> MGSSHHHHHHSSGLVPRGSHSEQKLISEEDLSMASISKDFTNLLNTLIDGQIGAASRQTEWFNMSPDERTDYIKQVDERLQEMQQSTLSVLAAQHFQMQDNPVSVGDQLQTLQKRRQQMTDVPGTPAINAYKQQLDRDILLYRRQQTAMTHFDSTWRKVLVMLGPDDSKPLNATTLRENAVDKQAKLDTEIKRLEQQLTIQVADSTFSQKYVTLFSELQAYKDVNARYNALLKASATEEAAALGALTKVPQASDDLPVNISLLMMEERPGYIRMNVALVNASTDGRFKDFFLENGRLVVLTDGVLNFSFGTAARSLAWQQQYRLKSEPPSFRSPTYTPIRSVLVKTEFVEKYFANYLVSESTLRGGFKAQLLGNGRKMLLTSVDRKVPNQIGIQVSGQAPNTTITREVPLASALSDLINQNADIASFRTIGLEGFRQSSYHPDRDGLFVNIHELERSVGFAGRQYLLEMPQDNDYLSATPFGVMSVDGDKVSSSHLSKAQTDTLYQYNAAFFEKLEQLRSGGMKASRLFEGSIERTAFVQQLVRLLERNHITPAGVLAPEYPRDNMRDIKGNNLNKVLWEQAFAASVWRSRDNDPLLFRLATRLVKNPAVVKVLQNGYVQSDIAQARELLAPLYEQWRTRAVEAETQRVASANAAQHPSNPKVHVFDQAEVERSLDDKLLILLLTGPQSLEGTDVQLRPMVEAALLSNEGRSLRKQILFHALRPVADSFSKAAAPVNPHAELGVGKIMINNRLNQPDPYLILNTSSEEQAYRDGSYLIKDDKYRSYNQFRPDFKNDATRYMNDLDTPFVGGISGTTQTVSNVLTELFGGALSVKQYWQFQMANAAFMIRNGYHSFFETFYVAARYEPEGADSIGKEMLQMFDKYRVEGSKKALQGKLYDGVMARVLPIINQGLSAADEFHPPRFTRIGPRPALLGQAVKDLELKAGLTSVGDGFEPRQGSADIHQFVTDPVLFAKTHTVSAEALVRSGRLPAEGSAQLVKVGSGLYELEYTEQSANDISSSSIPAYFLGYNGPNQANAVPAYVDIPKRTIAGNFLFTGTLSGGSLVVTSLDANTFRVYHDGRVNSSLLYDNVVMAVDYKDYQIAGTAEGLAAAYMQYVNHEWQLVLQRQEYQRDGQMLRLRLRDDEEPLSIQVADSQVVERNQAQFVAYREQIHQQLKKVATQFEVSISGVSDGVYTEGEFSPDHPAIAAWAKLCAEVYDRINADTKQLVDKRNKLYENRRNTIRRDLINQQIKQLNITLEYYKAQYDTVLREAGFVEQSWLWQQIKAKNGSAAVVRIDDTAIQGGGKQRTDSVGERYAISEAYQRGARGTGFSDGLRNFREIEIPGVDDKMSALEMKRLFLEGKLTSEQQGALSGRITETSRAEYIDKVLRQTAVFSEDFHDAGSVFDRLVPQDFYLSLVGDRSGGRCYPLVRAMTVALASGGEAGINSLVQKLFFASADPQAGSSTLLRNSLIKLHSNVEAVQASTELGQFGLSEVVSRLAATTGTSMFALNTQNHSMMVGSTVTTEGRRYYFYDPNVGIFAFDNTKSLSRAMEQHLVGRRLAVHYGSFGSKSAPAFNLIEIDTGKMAEVPVGNGLNVADLTRFEELSSVIGQRRQVEQVMSAQERITEDLQLSTALQAFDAEQWGARFEAASTRLAQEHQLDSRWLPIIATTEEQGEGRYRVQFINRDQPEQTRWLDTDDSTFVEFRRFVDEHMSVLNEHFTLESGRMRPRGGVGEAAPVDGLNAGFAVQALIQWFSDKNRHDAANGMASPDLATALKVHSYLNFVQMVHGGVQDVIKVTALVRTALRGEVVAAQTSFKEFALSLGHTVNEGVGVLFGGAMIGLDAYELAHAENDVQKAVFGTQLAFDSASFVTGAAGIGAGLVGASTAGAVLGGAGVILGGLAVGFTALAQAFGAVAEDAKAVGRYFDTVDKAYKGNGYRYDNEKQVLVPLAGAVIKTLDLSKNQIDFDSQYIYRTHSGSTGSGKINYFFWVGDFPRMVHDRGQAIEVRSGIGYKDVSRPLEHGDSNVVILPGTPKSYISYEYMLLPGATTRHDAGFDVIRRLEEDKRFDYDFYIFPGEETIRRIHHEYVDTPIEVVLDQRNRQLVAPELPKELHGFLCYEIKGAGGEYLIGLNEGAKVNLTSDVASTWIIDSSQLASDSISVSKDQLLVGEKGKEVVVKLYLAQNSQVLVVNGKGEVRKVDFTSLTAQVISEDASKWQVPGQQIEQHLSDLAKAHQLHGQYVVVENYRHQGRDVGRAFYDVTKDRMLFTDTTNEQAKRAQLGAVMGDYAYFYDADNAVAWRVDIATGQVDAQFEPWFNQNAGHISRFWQEGDVVYLARRYRLKEREAELGYRIIGDRMELVSAVGDDALLQLSARIGRHGDELEAILQGYRSNSTQRGTLMYTLGARLIQPTSAALVTVFGVDAAGVPHRYWIRTSDGTLIKPNLAPPADQTLHFEAHEQTRSAWQIPADLVLAGSMPLLGGKEVFFFYSKEQKTLFRQEGPGQEVLDANQPSALRVTTPALTNVINLNGHLVVVTEDGRVARLDALGQLSYAAVNEHWLKGRIHWWQDLTSVTDGRATLAVFGVKDTDGKSLLPVWYHNGQVVVASAALQDKHPQFLGFEVDGSSARLFEPASGKLYRQPAMTADALAAAFGTDEVLEASAQLPAANELEPELHLKAAEQVDAGLRLTTVKGEILLRTHDGKLQLVAVDKDWQQDNLVRLSQALAEVAGQWRVKGVLTLQGDDTQGWFDVGSGQVFSIGGIPATDNLRFIGIAVGKKGAYVYNPTDQMLYQVKESGAQKLNHYADVERIGSSLLLQDGGKGDLSPMLIAGVDSVVLHGGAGSDTYRLSQTMWSYYRTVVIDNDDPNQVLDRLIILAVDAEKIFVSRHEDDLMLTDSVNGTVLVIRKVFGSQAVTHRHLQIDLEGSSSVISVDHLVKGFTRLGTANIGLFELPWAIELDYKDDDDK

The bacterial Makes caterpillars floppy 1 (Mcf1) toxin promotes apoptosis in insects, leading to loss of body turgor and death. The structure reveals that Mcf1 is divided into an N-terminal head region and a C-terminal tail region. The head contains an N-terminal effector domain (NED), an activator-binding domain (ABD), and a protease effector domain (PED). The tail consists of two putative translocation and three putative receptor-binding domains.

To understand how Mcf1 is built in molecular detail, we heterologously expressed and purified the full-length Mcf1 complex from Photorhabdus luminescens and determined its structure using single particle cryo-EM to 3.6 Å resolution. Since the toxin proved to be inherently flexible, we performed a series of signal subtraction and local refinements of subregions of the complex. The resulting composite reconstruction allowed us to build 92% of the Mcf1 atomic model de novo. The structure reveals that Mcf1 is a monomeric, asymmetric protein. Based on its overall shape, reminiscent of a seahorse, it can be divided into two parts - an N-terminal head and a C-terminal tail region. In addition, we noticed a large spherical density of 10 Å diameter in the middle of the head that is coordinated by five arginines from all three head domains. Its location at the interface of the three domains and coordination suggests that this is a negatively charged molecule, which stabilizes the head region. We therefore call it head-stabilizing element (HSE). Interestingly, these putative receptor-binding domains are arranged such that they fold back onto the tail towards the head, resulting in the C-terminus of Mcf1 to be located within 2 nm distance from its N-terminus at the neck region. Moreover, the C-terminal region forms multiple hydrophobic interactions with a helix bundle of the ABD and supports the helix that directly connects the head and the tail region of the toxin, thus organizing the neck region.>[2x]GMSDEQHDSVWPPPGLDFSKPTIARVYDALLGGKDNFEADRALADYACKHIPGLKE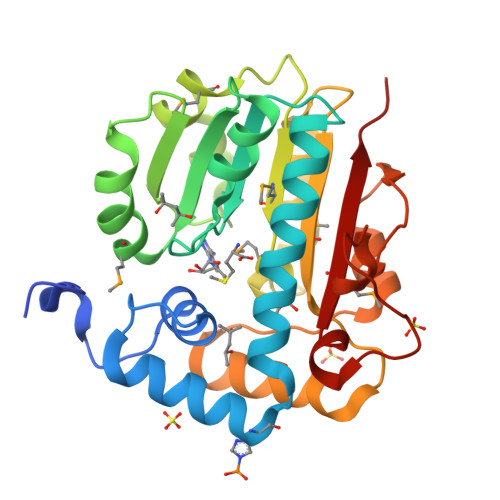SAIENRKVLVRGVRFLAGEAGISQFLDLGSGLPTVQNTHEVAQSVNPDARVVYVDIDPMVLTHGRALLAKDPNTAVFTADVRDPEYILNHPDVRRMIDFSRPAAIMLVGMLHYLSPDVVDRVVGAYRDALAPGSYLFMTSLVDTGLPAQQKLARITRENLGEGWARTPEEIERQFGDFELVEPGVVYTALWRPDEPVDPDNLSPGEQLGMAGIGRKKA>[2x]ARLGARPCGLRELEVRVSELGLGYASDE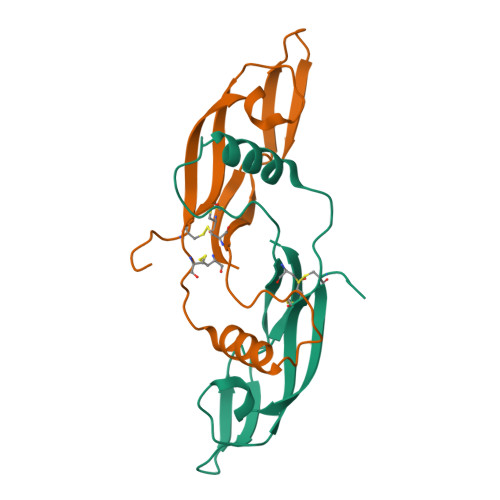TVLFRYCAGACEAAARVYDLGLRRLRQRRRLRRERVRAQPCCRPTAYEDEVSFLDAHSRYHTVHELSARECACV> MTSLEKARELLREFPVVDGHNDLPWALREQVRYDLDARDIAADQSAHLHTDLARLRSGGVGAQYWSVYVRSDLPGAVTATLEQIDCVRRLIDRHPGELRAALTAA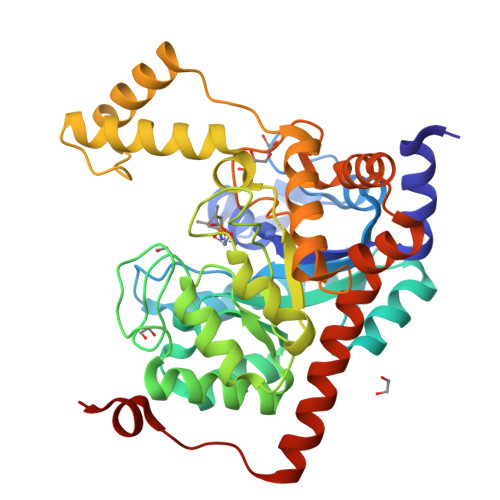DMEAARAEGRIASLMGAEGGHSIDNSLATLRALYALGVRYMTLTHNDNNAWADSATDEPGVGGLSAFGREVVREMNREGMLVDLSHVAATTMRDALDTSTAPVIFSHSSSRAVCDHPRNIPDDVLERLSANGGMAMVTFVPKFVLQAAVDWTAEADDNMRAHGFHHLDSSPEAMKVHAAFEERVPRPVATVSTVADHLDHMREVAGVDHLGIGGDYDGTPFTPDGLGDVSGYPNLIAELLDRGWSQSDLAKLTWKNAVRVLDAAEDVSRGLRAARGPSNATIEQLDGTAAEQPEG> SMAVEPKEDTITVTAAPAPQESAWGPAATIAARQSATGTKTDTPIQKVPQSISVVTAEEMALHQPKSVKEALSYTPGVSVGTRGASNTYDHLIIRGFAAEGQSQNNYLNGLKLQGNFYNDAVIDPYMLERAEIMRGPVSVLYGKSSPGGLLNMVSKRPTTEPLKEVQFKAGTDSLFQTGFDFSDSLDDDGVYSYRLTGLARSANAQQKGSEEQRYAIAPAFTWRPDDKTNFTFLSYFQNEPETGYYGWLPKEGTVEPLPNGKRLPTDFNEGAKNNTYSRNEKMVGYSFDHEFNDTFTVRQNLRFAENKTSQNSVYGYGVCSDPANAYSKQCAALAPADKGHYLARKYVVDDEKLQNFSVDTQLQSKFATGDIDHTLLTGVDFMRMRNDINAWFGYDDSVPLLNLYNPVNTDFDFNAKDPANSGPYRILNKQKQTGVYVQDQAQWDKVLVTLGGRYDWADQESLNRVAGTTD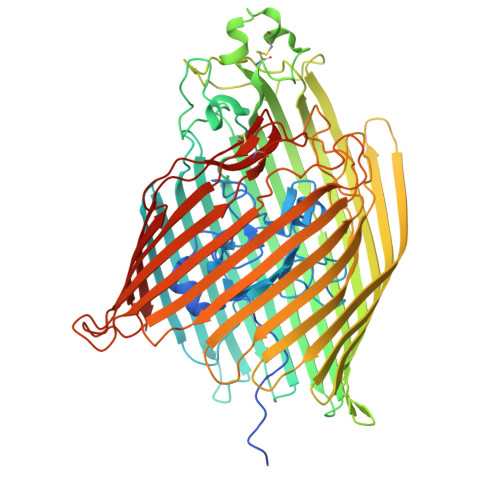KRDDKQFTWRGGVNYLFDNGVTPYFSYSESFEPSSQVGKDGNIFAPSKGKQYEVGVKYVPEDRPIVVTGAVYNLTKTNNLMADPEGSFFSVEGGEIRARGVEIEAKAALSASVNVVGSYTYTDAEYTTDTTYKGNTPAQVPKHMASLWADYTFFDGPLSGLTLGTGGRYTGSSYGDPANSFKVGSYTVVDALVRYDLARVGMAGSNVALHVNNLFDREYVASCFNTYGCFWGAERQVVATATFRF> MSSATKQFTLPDLLAMCPFTGST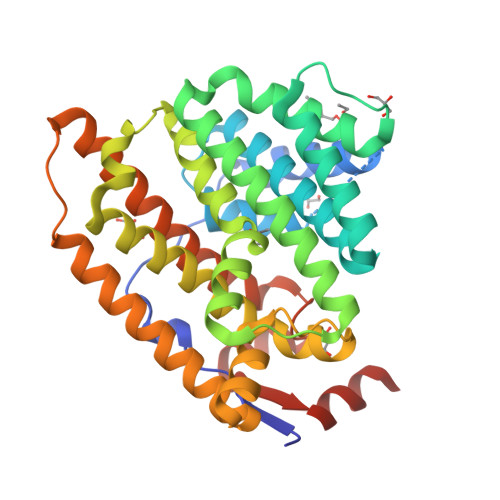NPHYAKAAAESSAWVNSYNILSDRKRAFFVTGSNELLVSHTYPYAGYEQFRTCCDFVNLLFVVDEVSDDQNGQDARQTGNVYLNAMRDPAWDDGSALAKMTKEFRARLLRYAGPGCYRRFLKHCEDYVDAVAREAEYRERGYVLDMASFETLRRENSAIRLCFGLFEYVLGVDLPEGVFEDPVFMTLYWAAADMVCWSNDVYSYNMEQAKGHSGNNIVTVLMRQKNVDLQTASDLVGEHFATLMDRFVTAKGGLPSWSPSVDAAVSDYVRAMEYWVTGNLEWSFETQRYFGVMHAEIKYTRLISLREREEEELEHHHHHH>[2x]GSGGSGKVVKFSYMWTINNFSFCREEMGEVIKSSTFSSGANDKLKWCLRVNPKGLDEESKDYLSLYLLLVSCPKSEVRAKFKFSILNAKGEETKAMES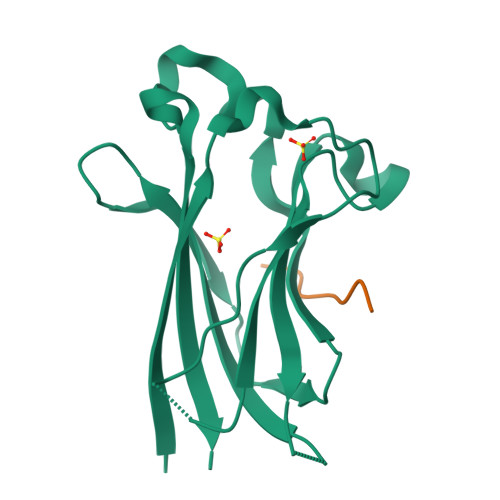QRAYRFVQGKDWGFKKFIRRGFLLDEANGLLPDDKLTLFCEVSVVQD;>NTLFPDVSSSTH[2x]> EDCQNLLKPCS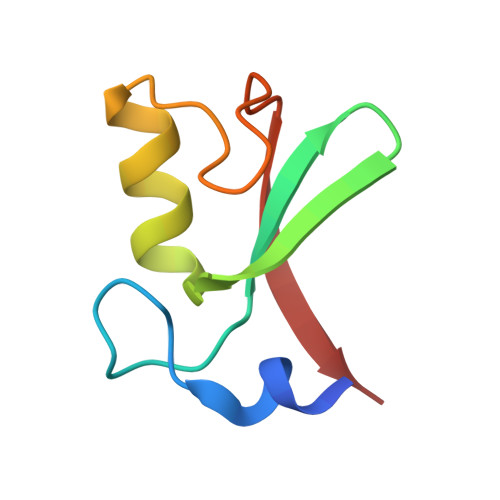LCEKRPRDGNIIHGRTGHLVTCFHCARRLKKAGASCPICKKEIQLVIKVFIA> GGCUUAUCAAGAGAGGGAGAGCGACUGGCGCGAAGAACCCCGGCAACCAGAAAUGGUGCCAAUUCCUGCAGCGGAAACGUUGAAAGAUGAGCCG

One especially common junction element is the kink-turn (k-turn). k-turns are elements in double-stranded RNA that introduce a tight kink into the helical axis, with an included angle close to 50°. A standard k-turn comprises a three-nucleotide bulge followed by successive G•A and A•G trans G(sugar edge)•A(Hoogsteen edge) basepairs. k-turns are commonly-occurring motifs that introduce sharp kinks into duplex RNA, thereby facilitating tertiary contacts. Both the folding and conformation of k-turns are determined by their local sequence. k-turns fall into two conformational classes, called N3 and N1, that differ in the pattern of hydrogen bonding in the core. We show here that this is determined by the basepair adjacent to the critical G•A pairs.

We therefore decided to extend the study with a systematic structural analysis of HmKt-7 as a function of the 3b,3n sequence. This was performed in the constant environment of the SAM-I riboswitch, modified by replacing its natural k-turn by HmKt-7 with different 3b,3n sequences. In this way we could observe the effect of changing the 3b,3n sequence alone in an otherwise completely unchanged RNA molecule. There is a tendency for 3b = purine to result in an N3 structure, but the generality is broken by the N1 structure adopted by the 3b,3n = G•G Kt-7 variant. Moreover, the structures of the HmKt-7 variants inserted into the SAM-I riboswitch demonstrate that changing the 3b,3n sequence is sufficient to switch the equilibrium conformation of the k-turn.>MKIEAITGSEAEAFHRMGSQASHRYDEFVDLLVGAGIADGQTVVDLCCGSGELEVILSSRFPSLNLVGVDLSEDMVRIAREYAAEQGKALEFRHGDAQLLAGMEDLAGKADLVVSRNAFHRLTRLPAAFDTMLRLAKPGGAVLNCSFIHPSDFDESGFRAWVTFLNQRPWDS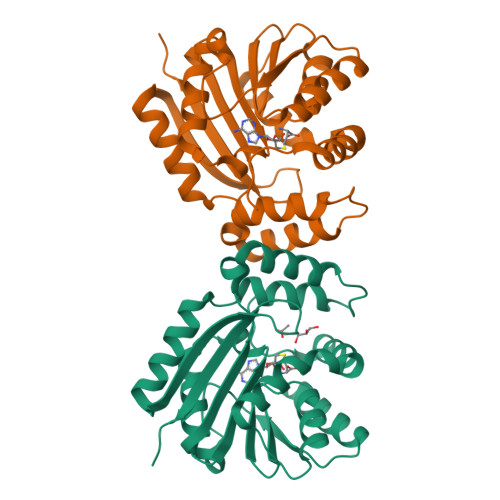EMQIVWALAHHYAPRLDDYREALAQAARETPVSEQRVWIDDQGYGVPTVKCFARRAAAHHHHHH[2x]> MHHHHHHSSGLEVLFQGPEFSGFLVSFMVDARGGAMRGCRHNGLRIIIPPRKCTAPTRVTCRLVKRHRLATMPPMVEGEGLASRLIEVGPSGAQFLGPVIVEIPHFAALRGKERELVVLRSENGDSWKEHFCDYTEDELNEILNGMDEVLDSPEDLEKKR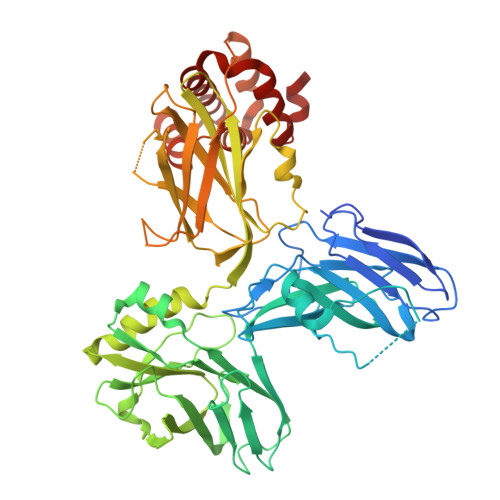ICRIITRDFPQYFAVVSRIKQDSNLIGPEGGVLSSTVVPQVQAVFPEGALTKRIRVGLQAQPMHSELVKKILGNKATFSPIVTLEPRRRKFHKPITMTIPVPKASGDAPTLRLLCSITGGTTPAQWEDITGTTPLTFVNECVSFTTNVSARFWLIDCRQIQESVTFASQVYREIICVPYMAKFVVFAKSHDPIEARLRCFCMTDDKVDKTLEQQENFAEVARSRDVEVLEGKPIYVDCFGNLVPLTKSGQHHIFSFFAFKENRLPLFVKVRDTTQEPCGRLSFMKEPKSTRGLVHQAICNLNITLPIYTKESESDQEQEEEIDMTSEKNPQDEQERIEERLAYIADHLGFSWTELARELDFTEEQIHQIRIENPNSLQDQSHALLKYWLERDGKHATDTNLVECLTKINRMDIVHLMETNT CD8 is expressed on the T-cell surface as dimers in two isoforms, the CD8αα homodimer and the CD8αβ heterodimer; both consist of an extracellular immunoglobulin variable (IgV) domain, a stalk region, a transmembrane domain and a cytoplasmic tail. Here, we report the high-resolution crystal structures of chicken, swine and bovine CD8α and confirm that they are capable of forming homodimers. All of them are CD8αα homodimers, and each CD8α exhibited a typical IgV architecture consisting of two anti-parallel sheets. Our results suggest that although CD8α and MHC I sequences change drastically during co-evolution, a few conserved key residues ensure that the CD8α forms dimers and interacts with p/MHC I during at least the co-evolution of endotherm species.

Three extracellular Ig-like domains of chicken, swine and bovine CD8α (cCD8α, sCD8α and bCD8α) were crystallized and diffracted to 2.0 Å, 1.8 Å and 1.8 Å, respectively. The sheets of CD8α are composed of 10 β strands, but there are 11 β strands in sCD8α and bCD8α because their A and G strands are divided into two separate parts. The two artiodactyl CD8αα dimers also have some distinct structural characteristics, and the most notable feature is that they have an additional A’ strand. The two artiodactyl sCD8αα can be discriminated from each other by certain characteristics, such as the longer A’ strand and shorter complementarity determining region 2 (CDR2) loop in sCD8αα. There was a special helix and a short CDR2 loop found in cCD8αα, and the inter-chain hydrogen bonds and the dimer interface area of cCD8αα were minimal. sCD8αα and bCD8αα showed an additional A’ strand, but the A’ strand in sCD8αα was longer. The buried surface areas (BSAs) of cCD8αα, sCD8αα, bCD8αα, mouse CD8αα (mCD8αα), rhesus macaque CD8αα (rCD8αα) and human CD8αα (hCD8αα) are 828.3 Å2, 979.6 Å2, 928.7 Å2, 1048.7 Å2, 1105.5 Å2 and 1026.3 Å2, respectively, indicating that they are tightly binding dimers. The BSAs of sCD8αα and bCD8αα are similar, but there are six hydrogen bonds in sCD8αα and only two hydrogen bonds in bCD8αα, indicating that CD8α dimerization does not mainly rely on hydrogen bonds. Especially for chicken, the four conserved aromatic residues contribute 161 VDW and 262.21 Å2 BSA, which account for 42% and 34% of the total VDW and BSA, respectively. These four aromatic residues can interact with each other; for example, F48 contacts F104 in sCD8αα as well as in other CD8αα. The numbers of residues composing the cCD8αα, sCD8αα and bCD8αα cavities are 7, 7 and 9, and their volumes are 202.0 Å3, 322.9 Å3 and 384.6 Å3, respectively.

>SLFRTSPEMVQASLGETVKLRCEVMHSNTLTSCSWLYQKPGAASKPIFLMYLSKTRNKTAEGLDTRYISGYKANDNFYLILHRFREEDQGYYFCSFLSNSVLYFSNFMSVFLPA[2x]> MPDSGQLGAADTPLRLLSSVHYLTDGELPQLYDYPDDGTWLRANFISSLDGGATVDGTSGAMAGPGDRFVFNLLRELADVIVVGVGTVRIEGYSGVRMGVVQRQHRQARGQSEVPQLAIVTRSGRLDRDMAVFTRTEMAPLVLTTTAVADDTRQRLAGLAEVIACSGDDPGTVDEAVLVSQLAARGLRRILTEGGPTLLGTFVERDVLDELCLTIAPYVVGGLARRIVTGPGQVLTRMRCAHVL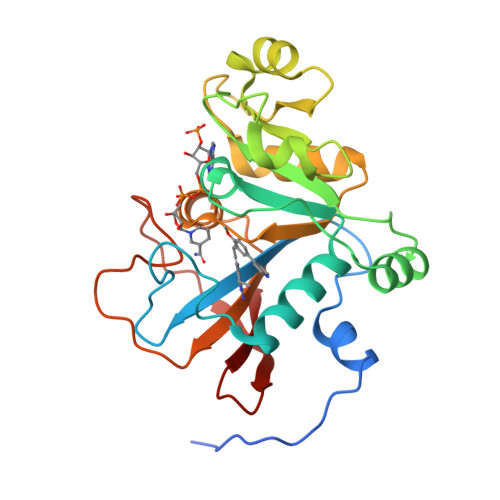TDDSGYLYTRYVKT> MSYSKDIVLEKLASLEETQISIQSIGQWCLFHHRHAPETVAIWSEFVGSTQTKKLAGLYLANEIIQQSRAKRKTTF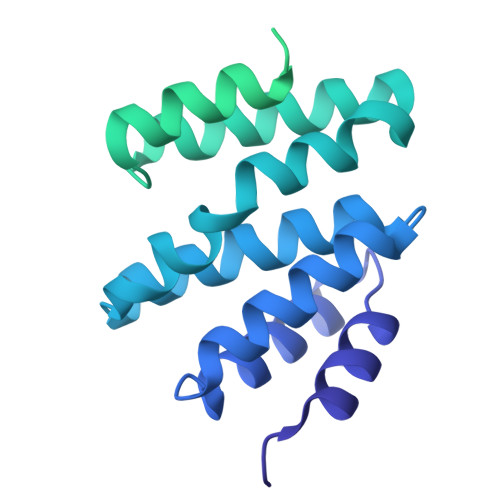LDEFAKVLPSTLEQIYPSMISTHQAKLKRIIDVWSQRKIFDSNLIHRLYQSIQDQKAYNGLSSSSSNSPPINSGDLAPEISSLSTLFNKISTLKSSTSLVVNQINEQYSSLFDSETLPGTDIYLKQLGDLSTLITSARSKSQETQELRESIINELKKLIQVQESWITKDAESSGSLDEKLATVQQKESELKEFINDVEEEDGVPQYAASSDEEGDENVSKKRKMESPPTETVDSGEQPTNPVHPQLSSILESLSRTTGLTPEPASTSDESATATQKQDETPVSSSINPALASLLSKLNGLEVLFQ>MHHHHHHAIKLIVGLANPGAEYAATRHNAGAWYVDLLAERLRAPLREEPKFFGYTSRITLEGEDVRLLVPTTFMNLSGKAVGAMASFYRIQPDEILVAHDELDLPP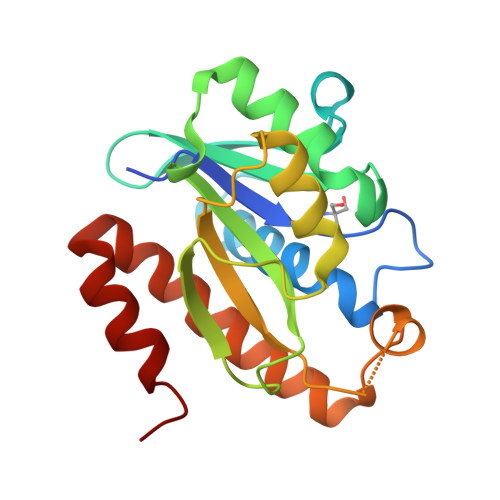GVAKFKLGGGHGGHNGLKDIISKLGNNPNFHRLRVGIGHPGDKNKVVGFVLGKPPVSEQKLIDEAIDEAARCTELWFKEGLAKATSRLHTFKAQ[2x]>[2x]HMNAEINPLHAYFKLPNTVSLVAGSSEGETPLNAFDG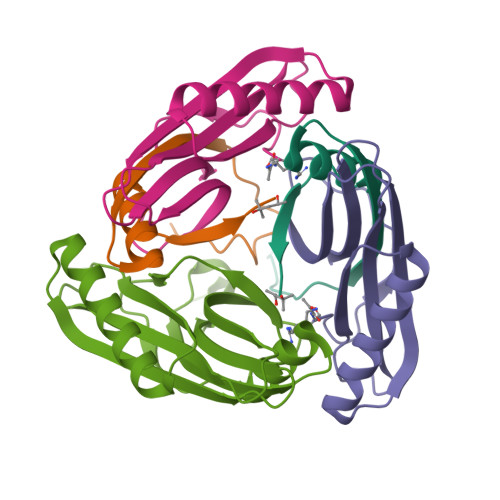ALLNAGIGNVALIRIS;>[2x]IMPPEAEIVPLPKLPMGALVPTAYGYIISDVPGETISAAISVAIPKDKSLCGLIMEYEGKCSKKEAEKTVREMAKIGFEMRGWELDRIESIAVEHTVEKLGCAFAAAALWYK;>[4x]HMNAEINPLHAYFKLPNTVSLVAGSSEGETPLNAFDGALLNAGIGNVALIRISSIMPPEAEIVPLPKLPMGALVPTAYGYIISDVPGETISAAISVAIPKDKSLCGLIMEYEGKCSKKEAEKTVREMAKIGFEMRGWELDRIESIAVEHTVEKLGCAFAAAALWYK> MLKGKKAVVTGSTSGIGLAMATELAKAGADVVINGFGQPEDIERERSTLESKFGVKAYYLNADLSDAQATRDFIAKAAEALGGLDILVNNAGIQHTAPIEEFPVDKWNAIIALNLSAVFHGTAAALPIMQKQGWGRIINIASAHGLVASVNKSAYVAAKHGVVGLTKVTALENAGKGITCNAICPGWVRTPLVEKQIEAISQQKGID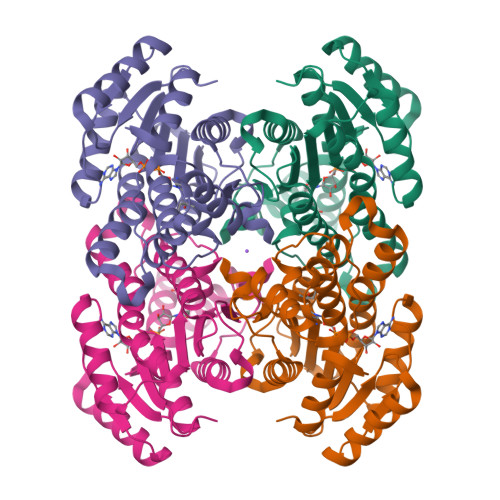IEAAARELLAEKQPSLQFVTPEQLGGAAVFLSSAAADQMTGTTLSLDGGWTAR> MPSGTDDPLSDAEIQKYREEINRLDREILDAVKRRTKISQTIGKTRMSSGGTRLVHTR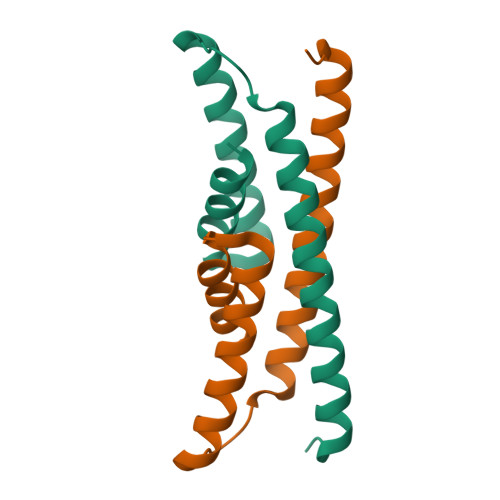EVAIINQFREEIGEEGPALAGILLRMGRGKLG>GGGCGCCC[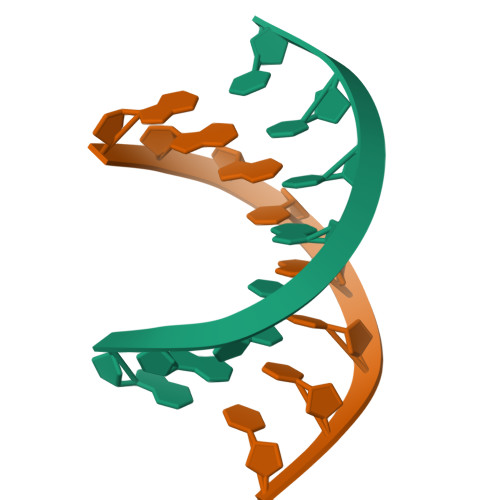2x]In this report we present 11 diffraction data sets, in multiple space groups, from the E. coli enzyme N-acetyl-neuraminic acid lyase (NAL), which present twin lattices and incommensurate modulation. NAL crystallised in four different crystal forms from the same crystallisation conditions, and in the same drops (100 mM Tris-HCl pH 8.0–8.2, 200 mM Na acetate, 18–22% w/v PEG3350). The development of twin refinement in REFMAC, which at the time was only implemented in the experimental version of the program, allowed the determination of several apo- and ligand bound structures of NAL and the proposal of the first detailed mechanism of the enzyme reaction.

Interestingly, the three crystal forms in space group P21 were not related to each other, two of them were twinned and shared the same twinning operator, which made the monoclinic cells a pseudo-orthorombic cell. With the P21 indexing choice, POINTLESS initially assigned the space group C2221 but reflections belonging to one of the 2-fold axes were much stronger than the others (data not shown), which is consistent with pseudo-merohedral twinning in P21, and indeed with this choice the structures could be easily solved. Although they could all be solved by molecular replacement, they could not be refined satisfactorily using standard protocols. As a general rule, whenever only a single lattice with no incommensurate modulation was present, indexing, data reduction and molecular replacement were possible, but the (non-twin) refinement stalled at Rfactor and Rfree values of 30–35% for all datasets (resolution range 1.45–2.3 Å, <I/σ(I)> cut off = 2.0) where we would expect Rfactor values near or below 20% for well-behaved refinements. Refinement with the program REFMAC (versions 5.6 and 5.7) identified the twinning operator (−h, −k, h + l) for all the cases, in which twinning was detected. Twin refinement resulted in improved models with Rfactor and Rfree values ~18–20% (data collection and final refinement statistics are summarised in Table 1). Inspection of the packing using the molecular graphics program COOT25 highlighted how not only the inter-monomer contacts within the NAL tetramers were different, but also the inter-tetramer contacts in the crystal lattice. We speculate that the likelihood of NAL of crystallising in any one of the four forms is determined by small differences in the interfaces between tetramer during nucleation and the early stages of crystal growth.

>[4x]MEHHHHHHATNLRGVMAALLTPFDQQQALDKASLRRLVQFNIQQGIDGLYVGGSTGEAFVQSLSEREQVLEIVAEEAKGKIKLIAHVGCVSTAESQQLAASAKRYGFDAVSAVTPFYYPFSFEEHCDHYRAIIDSADGLPMVVYNIPALSGVKLTLDQINTLVTLPGVGALKQTSGDLYQMEQIRREHPDLVLYNGYDEIFASGLLAGADGGIGSTYNIMGWRYQGIVKALKEGDIQTAQKLQTECNKVIDLLIKTGVFRGLKTVLHYMDVVSVPLCRKPFGPVDEKYLPELKALAQQLMQERG> MALLWQLARNAEGDDPTNLESALIGKPVPKFRLESLDNPGQFYQADVLTQGKPVLLNVWATWCPTCRAEHQYLNQLSAQGIRVVGMNYKDDRQKAISWLKELGNPYALSLFDGDGMLGLDLGVYGAPETFLIDGN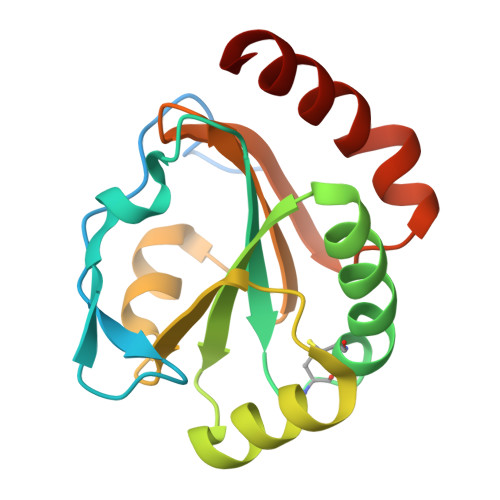GIIRYRHAGDLNPRVWEEEIKPLWEKYSKEAAQ>MAKIYLASPFFNEEQLKHVSKAEQVLRDLGHTVFSPRENQLPEVEFGSFEWRTFVFKNDLEHIKWADITFGIIGDNYDDTGTAWELGASYILGKPVMLFSPTGEIINLMI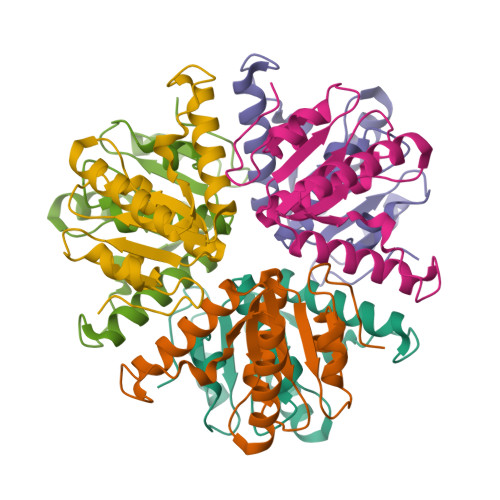TDSLHAYFEDWNDVENYDFATLPIKPYLKAVK[2x]> MAHHHHHHMNPHPVEPRD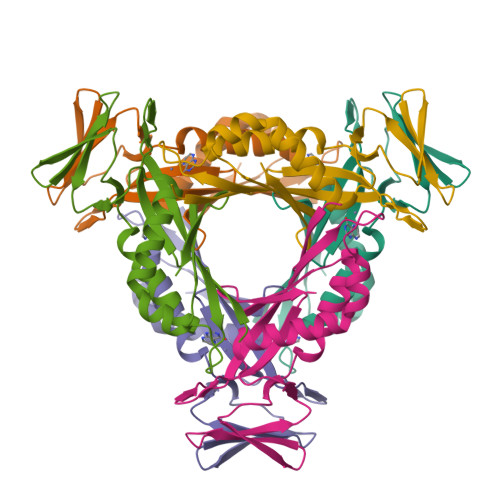QIAELLVESPLFSFNCAHFIAFKGFRCTLHGHNYNVSLRLRGNIQGDGYVIDFSILKEKVRKVCKQLDHHFILPMYSDVLNIQEVNDNFKITCEDNSEYSFPKRDCVQIPIKHSSTEEIGLYILNQLIEEIDLPFLKTRSVNYMEVTVSESPSQKATVHRNI>MAHHHHHHMNALEHQLDYPFADTLPAAGDTFEVAPGVRWLRMPLPFSLDHINLWLLRDEIDGQAGWTVVDCGIASDAIRTHWEQIFDAHLDGLPVLRVIVTHCHPDHFGLANWLCEGGDKRRWNVRLWMTLGEYMFGCLMAAGNGSNAGGAAAADHFARHGLTDAASLEKLRNRRSYYSDLVPAVPPRYRRLRDGDAVTIGTRTWRVVTGYGHSPEHCALHSEADGVLISGDMVLPRISTNVSVFDLEPEANPLALYLQSLGRYETMAPDTLVLPSHGKPFRGVRTRIAQLRAHHDARLDEVRVACAEQPMSAADIVPIMFRRRELDIHQMTFALGEAIAHLN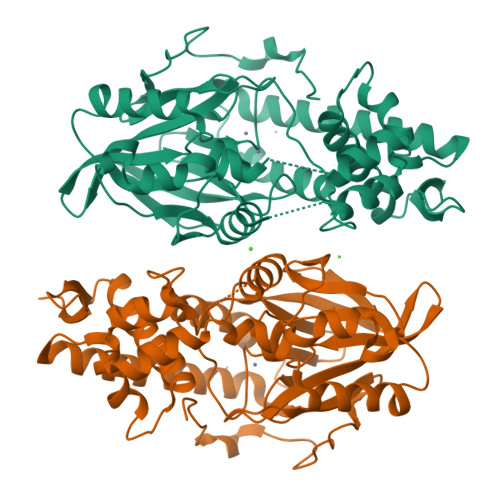LLWLAGELVREQGDDGVLRFRIAR[4x]> MMYIQVLGSAAAGGFPQWNCNCVNCKGYRDGTLKATARTQSSIALSDDGVHWILCNASPDIRAQLQAFA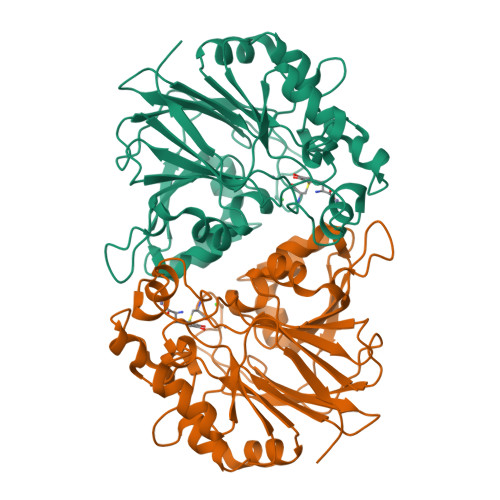PMQPARALRDTGINAIVLLDSQIDHTTGLLSLREGCPHQVWCTDMVHQDLTTGFPLFNMLSHWNGGLQWNRIELEGSFVIDACPNLKFTPFPLRSAAPPYSPHRFDPHPGDNLGLMVEDTRTGGKLFYAPGLGQVDEKLLAMMHGADCLLVDGTLWEDDEMQRRGVGTRTGREMGHLAQNGPGGTLEVLDGFPRQRKVLIHINNTNPILDENSPERAEVLRRGVEVAFDGMSIELLEHH N~4~-[7-(1-benzofuran-2-yl)-1H-indazol-5-yl]pyrimidine-2,4-diamine | C19 H14 N6 O | 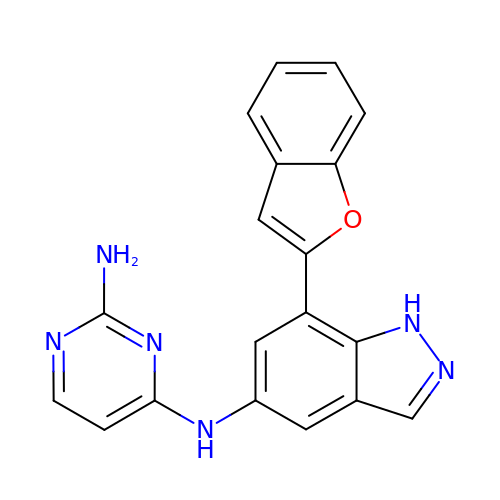IQDDLNJTLVXFQA-UHFFFAOYSA-N>AVPIAQKSEPHSLSSEALMRRAVSLVTDSTSTFLSQTTYALIEAITEYTKAVYTLTSLYRQYTSLLGKMNSEEEDEVWQVIIGARAEMTSKHQEYLKLETTWMTAVGLSEMAAEAAYQTGADQASITARNHIQLVKLQV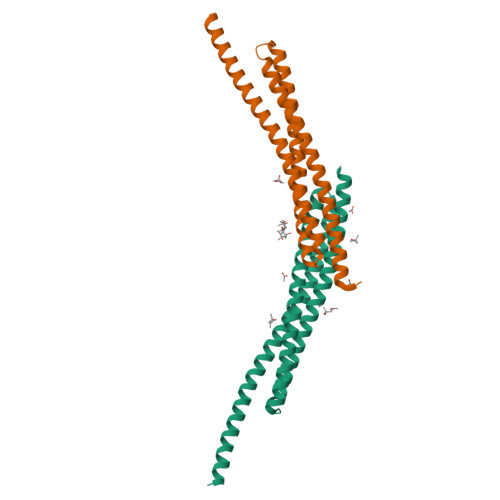EEVHQLSRKAETKLAEAQIEELRQKTQEEGEERAESEQEAYLREDLEHHHHHH[2x]1,3-BIS(AMIDINOPHENOXY)PROPANE 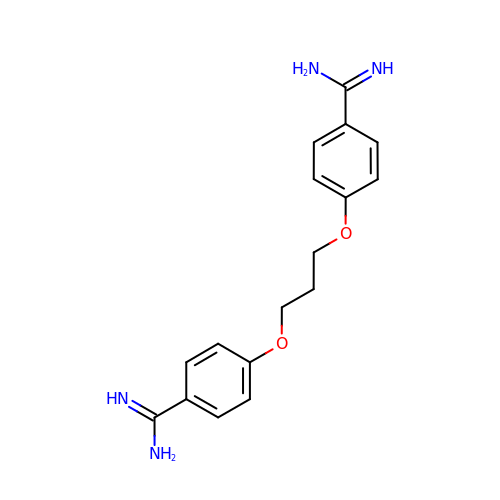| C17 H20 N4 O2 | WTFXJFJYEJZMFO-UHFFFAOYSA-N(R)-5-(8-CHLOROISOQUINOLIN-3-YLAMINO)-3-(1-(DIMETHYLAMINO)PROPAN-2-YLOXY)PYRAZINE-2-CARBONITRILE 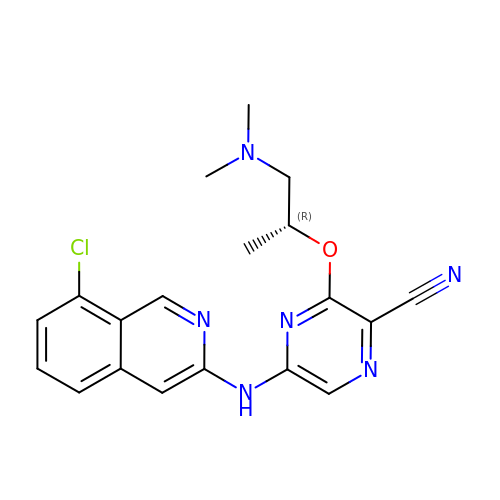| C19 H19 Cl N6 O | SRBJWIBAMIKCMV-GFCCVEGCSA-N>[3x]MRCVGVGNRDFVEGLSGATWVDVVLEHGGCVTTMAKNKPTLDIELQKTEATQLATLRKLCIEGKITNITTDSRCPTQGEAVLPEEQDQNYVCKHTYVDRGWGNGCGLFGKGSLVTCAKFQCLEPIEGKVVQYENLKYTVIITVHTGDQHQVGNETQGVTAEITPQASTTEAILPEYGTLGLECSPRTGLDFNEMILLTMKNKAWMVHRQWFFDLPLPWASGATTETPTWNRKELLVTFKNAHAKKQEVVVLGSQEGAMHTALTGATEIQNSGGTSIFAGHLKCRLKMDKLELKGMSYAMCTNTFVLKKEVSETQHGTILIKVEYKGEDAPCKIPFSTEDGQGKAHNGRLITANPVVTKKEEPVNIEAEPPFGESNIVIGIGDNALKINWYK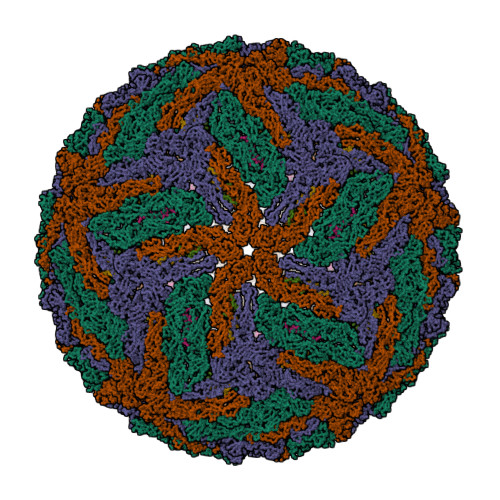KGSSIGKMFEATARGARRMAILGDTAWDFGSVGGVLNSLGKMVHQIFGSAYTALFSGVSWVMKIGIGVLLTWIGLNSKNTSMSFSCIAIGIITLYLGAVVQA;>SVALAPHVGMGLDTRTQTWMSAEGAWRQVEKVETWALRHPGFTILALFLAHYIGTSLTQKVVIFILLMLVTPSMT[3x]> MDQSSHHHHHHMDQKQIEEIVRSVMASMGQAAPAPSEAKCATTNCAAPVTSESCALDLGSAEAKAWIGVENPHRADVLTELRRSTVARVCTGRAGPRPRTQALLRFLADHSRSKDTVLKEVPEEWVKAQGLLEVRSEISDKNLYLTRPDMGRRLCAEAVEALKAQCVANPDVQVVISDGLSTDAITVNYEEILPPLMAGLKQAGLKVGTPFFVRYGRVKIEDQIGEILGAK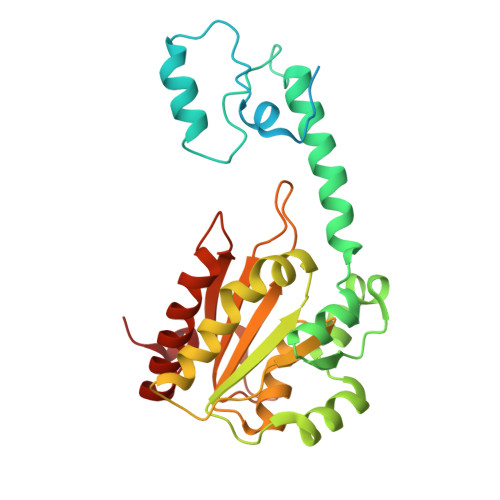VVILLVGERPGLGQSESLSCYAVYSPRMATTVEADRTCISNIHQGGTPPVEAAAVIVDLAKRMLEQKASGINMTR>MARRILVVEDEAPIREMVCFVLEQNGFQPVEAEDYDSAVNQLNEPWPDLILLDWMLPGGSGIQFIKHLKRESMTRDIPVVMLT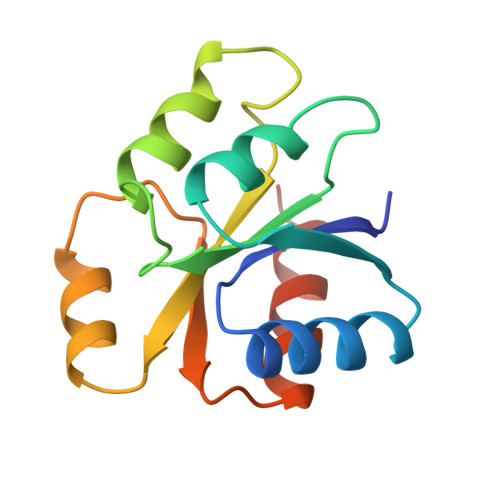ARGEEEDRVRGLETGADDYITKPFSPKELVARIKAVMRRISPMA[2x]> MEEPDANGYYYHDTFEGSVGQWTAAGPAEVLLSGRTAYKGSESLLVRNRTAAWNGAQRALNPRTFVPGNTYCFSVVASFIEGASSTTFCMKLQYVDGSG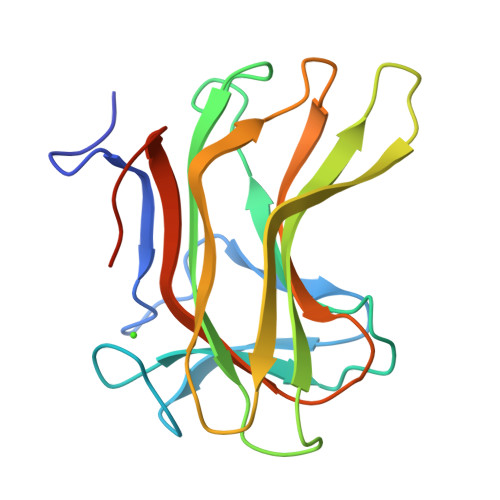TQRYDTIDMKTVGPNQWVHLYNPQYRIPSDATDMYVYVETADDTINFYIDEAIGAVAGTVIEGLEHHHHHH>GPAMKKLKPAPFYFQPFSKKQLKVLTWWRKASPVSDKDGIICDGSIRAGKTIVMSFSYVMWAMDTFNEQNFGMAGKTIGALRRNVITPLKRMLKSRGYRVKDHRADNYLTITFKGKTNYFYLFGGKDESSQDLIQGITLAGMFFDEVALMPESFVNQATARCSVDGAKLWFNCNPAGPYHWFKVEYLDKLDEKNLLHLHFTMDDNLSLSKQVKERYQRMYKGVFYQRYILGLWVLAEGIIYDMFDQDEHVVPTVPRPYEKYYVSCDYGTQNPTTFGLWGLYNGVWYKVKEYHYDGRKENK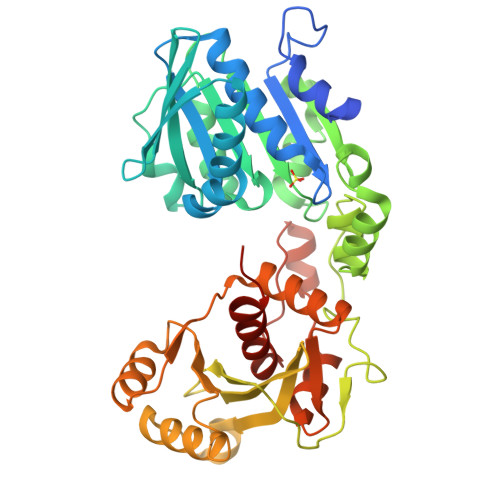QKTDQEYYEDLMKFIEDIEKHKFKGVIVDPSAASFIALLRQKGIKVIKAKNDVLDGIRNVATALNKKMILYNDCCKETFREYSSYVWDEKAAERGEDKPVKQNDHQLDADRYFVNTILFGNKLRAVPSLY[3x]> METRDDFMFELSDKPLLPCYNLQVSVSRGPCNWFLFSDVLKRLKLSSRIFQARFPHFEITTMPKAEFYRQVASSQLLTPAERPGGLDDRSPPG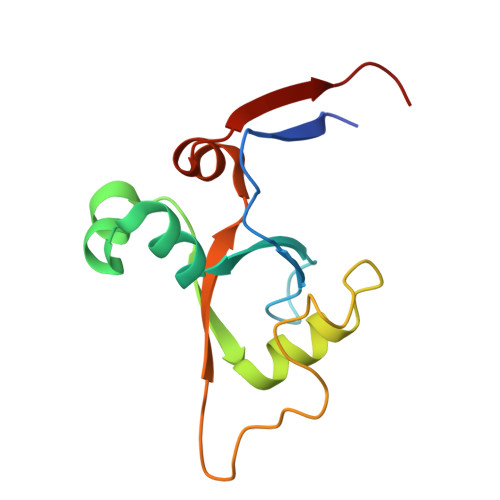SSETVELVRYEPDLLRLLGSEVEFQSCNS> GADDVVDSSKSFVMENFSSYHGTKPGYVDSIQKGIQKPKSGTQGNYDDDWKGFYSTDNKYDAAGYSVDNENPLSGKAGGVVKVTYPGLTKVLALKVDNAETIKKELGLSLTEPLMEQVGTEEFIKRFGDGASRVVLSLPFAEGSSSVEYINNWEQAKALSVELEINFETRGKRGQDAMYEYMAQACAGNRVRRSVGSSLSCINLDWDVIRDKTKTKIESLKEHGPIKNKMSESPNKTVSEEKAKQYLEEFHQTALEHPELSELKTVTGTNPVFAGANYAAWAVNVAQVIDSETADNLEKTTAALSILPGIGSVMGIADGAVHHNTEEIVAQSIALSSLMVAQAIPLVGELVDIGFAAYNFVESIIN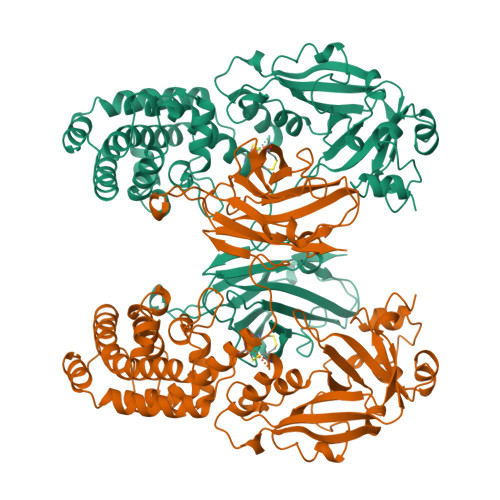LFQVVHNSYNRPAYSPGHKTQPFLHDGYAVSWNTVEDSIIRTGFQGESGHDIKITAENTPLPIAGVLLPTIPGKLDVNKSKTHISVNGRKIRMRCRAIDGDVTFCRPKSPVYVGNGVHANLHVAFHRSSSEKIHSNEISSDSIGVLGYQKTVDHTKVNSKLSLFFEIKS> LTAKHRPSVVWLHNAECGGCTEAAIRTIKPYIDALILDTISLDYQETIMAAAGEAAEAALHQALEGKDGYYLVVEGGLPTIDGGQWGMVAGHPMIETTKKAAAKAKGIICIGTCSAYGGVQKAKPNPSQAKGVSEALGVKTINIPGCPPNPINFVGAVVHVL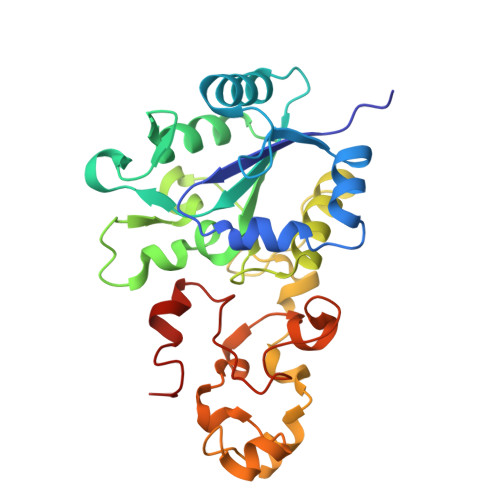TKGIPDLDENGRPKLFYGELVHDNCPRLPHFEASEFAPSFDSEEAKKGFCLYELGCKGPVTYNNCPKVLFNQVNWPVQAGHPCLGCSEPDFWDTMTPFYEQG>[4x]MKFLDQEKRRQLLNERHSCKMFDSHYEFSSTELEEIA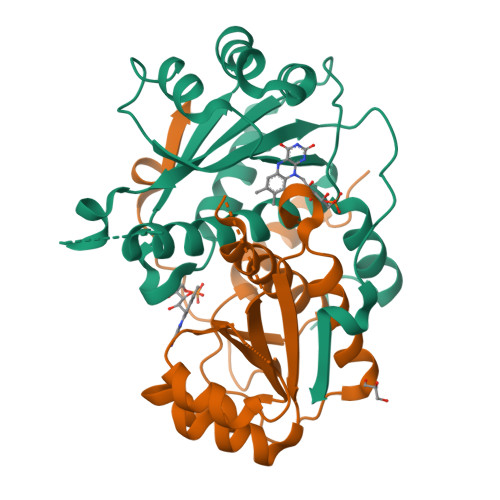EIARLSPSSYNTQPWHFVMVTDKDLKKQIAAHSYFNEEMIKSASALMVVCSLRPSELLPHGHYMQNLYPESYKVRVIPSFAQMLGVRFNHSMQRLESYILEQCYIAVGQICMGVSLMGLDSCIIGGFDPLKVGEVLEERINKPKIACLIALGKRVAEASQKSRKSKVDAITWL> PAKLGYWKLRGLAQPVRLFLEYLGEEYEEHLYGRDDREKWMSEKFNMGLDLPNLPYYIDDKCKLTQSVAIMRY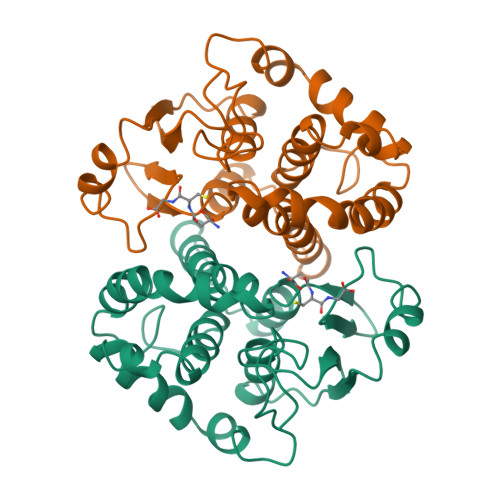IADKHGMLGTTPEERARISMIEGAAMDLRIGFGRVCYNPKFEEVKEEYVKELPKTLKMWSDFLGDRHYLTGSSVSHVDFMLYETLDSIRYLAPHCLDEFPKLKEFKSRIEALPKIKAYMESKRFIKWPLNGWAASFGAGDAPPS~{N},1-dimethyl-5-[[4-[3-methyl-4-[[(3~{R})-pyrrolidin-3-yl]amino]pyrazol-1-yl]pyrimidin-2-yl]amino]indazole-3-carboxamide | C22 H26 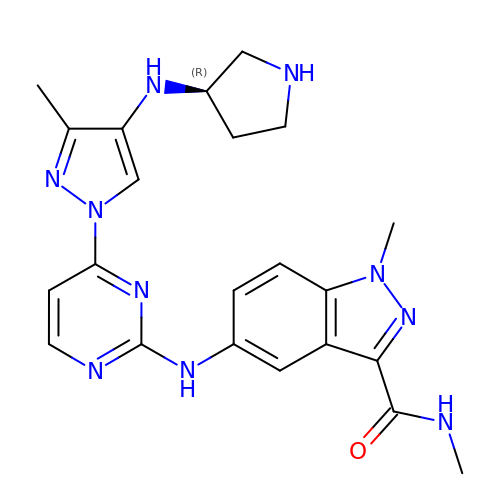N10 O | APXVIACNUKLHFZ-OAHLLOKOSA-N> GAMGSYDWLPRLSKENFNAAPVTCFPHAPGCEVWDNLGVGMKVEVENTDCDSIEVIQPGQTPTSFWVATILEIKGYKALMSYEGFDTDSHDFWVNLCNAEVHSVGWCATRGKPLIPPRTIEHKYKDWKDFLVGRLSGARTLPSNFYNKINDSLQSRFRLGLNLECVDKDRISQVRLA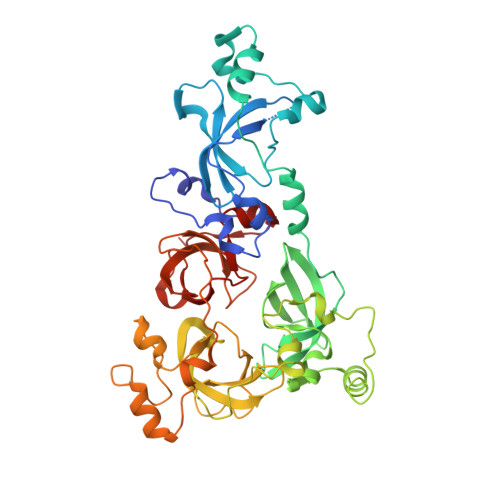TVTKIVGDRLFLRYFDSDDGFWCHEDSPIIHPVGWATTVGHNLAAPQDYLERMLAGREAMIEVHEDDATIELFKMNFTFDEYYSDGKTNSFVEGMKLEAVDPLNLSSICPATVMAVLKFGYMMIRIDSYQPDASGSDWFCYHEKSPCIFPAGFCSVNNISVTPPNGYDSRTFTWEGYLSDTGAVAAGQHLFHDIIPDHGFEVGMSLECADLMDPRLVCVATVARVVGRLLKVHFDGWTDEYDQWLDCESADIYPVGWCVLVNHKLEGPPR> HHHHHHNMAEKDDTAQVVVNNNDPTYKSEHTDTLVYNPEGALSYRLIAQHVEYYSDQAVSWFTQPVLTTFDKDKIPTWSVKADKAKL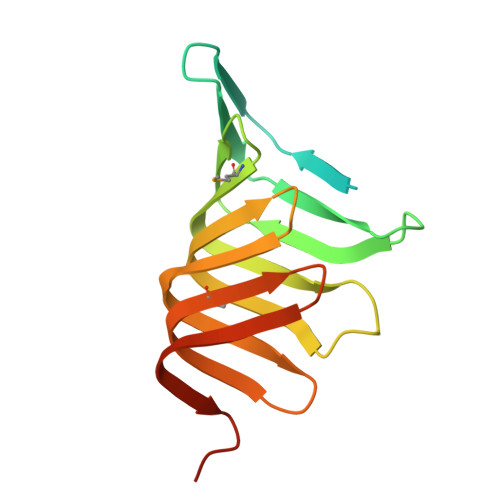TNDRMLYLYGHVEVNALVPDSQLRRITTDNAQINLVTQDVTSEDLVTLYGTTFNSSGLKMRGNLRSKNAELIEKVRTSYEIQNKQTQP> GSVAYHQKHGGYGRGGYG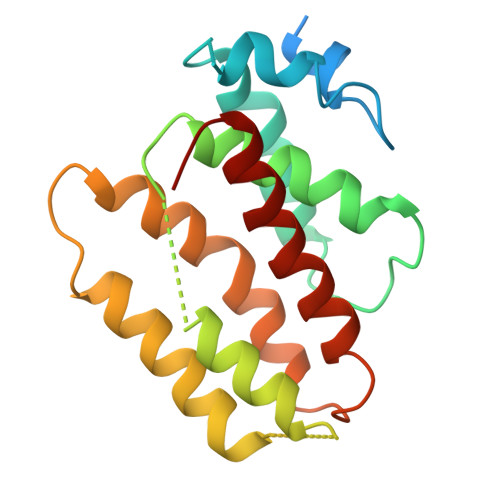RQDRPQVDASRLFGESPDVVGIKKMLEGKGKQWEAIQPYFDNVVREAKNFLEWSPNKRLANAVTVAAYLTSQGLKTNQVRKILDMARTTELKVKRGEGDIKDDLVKMRYLLAYTVGKATGQSKYSLDAFHRILDPMLEVLMGSPKKENFEKFYDFLQAVVAYHKFFGGGD The sliding clamp PCNA (proliferating cell nuclear antigen) is a central player in multiple aspects of chromosomal DNA replication, repair and genome stability. This ring-shaped homotrimer encircles double-stranded DNA to act as a processivity factor for DNA polymerases and a landing pad for the assembly of various DNA processing factors such DNA ligase I, the flap endonuclease Fen1, and the clamp loader complex replication factor C (RF-C) which opens and closes the PCNA ring around dsDNA. Many of the proteins that interact with PCNA, including DNA polymerase δ, DNA ligase I, Fen1 and RF-C, do so via a common mechanism that involves a short linear interaction motif on the partner protein called a PCNA-interacting protein (PIP) motif. The best characterised PIP motifs have conserved sequence Qxxψxxθθ, where ψ and θ represent amino acids with hydrophobic and aromatic side chains, respectively, but other variations on this sequence (so-called non-canonical PIP motifs) have been identified such as ψxxxθ and Qxxψxθ.

Fen1 is a 5’ flap-specific nuclease that plays an important in Okazaki fragment maturation. Key catalytic residues in human Fen1 are conserved in the C. thermophilum enzyme, as is the PIP motif located towards the C-terminal end of the protein (sequence: 342 QARIEGFF 349 with conserved PIP motif residues underlined). The Ct Fen1 PIP peptide-Ct PCNA structure was solved to a resolution of 1.95 Å. 14 of 15 residues in the Ct Fen1 PIP peptide were visible in the structure, revealing a 310 helix and the anticipated canonical binding mode, with Ct Fen1 Gln342 inserting into the Q-pocket, and Ile345 and Phe349 forming the two-fork plug that inserts into the hydrophobic surface pocket on Ct PCNA. As with Ct PolD3, the Ct Fen1 Q-pocket glutamine, Gln342, interacts with Ser208 and Ala252 in Ct PCNA, with the interaction with Ser208 involving water-mediated hydrogen bonding between Gln342 (OE1) and Ser208 (N), as is the case for the equivalent Gln441-Ser208 pairing in Ct PolD3, whereas the interaction with Ala252 involves a direct H-bond between Gln342 (NE2) and Ala252 (O), different from the water-mediated Gln441-Ala252 interaction in the Ct PolD3-Ct PCNA structure. Additional direct hydrogen-bonding interactions are seen involving Gln341 (N) and Ile255 (O), Gln341 (O) and Ile255 (N), Ala343 (N) and Pro253 (O), Ile345 (N) and His44 (O), Glu346 (OE2) and His44 (ND1), Lys350 (O) and Gly127 (N), and Ile353 (N) and His125 (O). In addition to this, the higher resolution of the structure allowed identification of multiple water-mediated hydrogen bonds connecting the Ct Fen1 peptide to Ct PCNA. A salt bridge links Glu346 (OE1) and His44 (ND1) also. As with the Ct PolD3-Ct PCNA structure, the 2-fork plus residues Ile345 and Phe349 display hydrophobic interactions with the surface pocket on Ct PCNA although in the case of Phe349 only a single interaction (involving Phe349 (CE1)) is apparent within the 3.9 Å length cut-off applied in the analysis.

> GAMALEARLEQASILKKVVDAIKDLVQDCNFDCNDSGIALQAMDNSHVALVSMMLKAEGFSPYRCDRNIALGVNLTSLTKVLRAAQNEDILTLKAEDAPDVLNLVFESSETDRISEYDLKLMDIDQEHLGIPETEYAATITMPSNEFKRITTDLMAMSESVTIEANKDGVKFSCQGDIGNGSVTLRQHTNVEKPNESIEIELSEPVSLTFSLKYLVNFCKASALSNTVKICLSNEVPLLVEYSLGGSSYLRFYLAPKIGDDE;> GAQQARIEGFFKVIP> DPPAPLPLVIWHGMGDSCCNPLSMGAIKKMVEKKIPGIHVLSLEIGKTLREDVENSFFLNVNSQVTTVCQILAKDPKLQQGYNAMGFSQGGQFLRAVAQRCPSPPMVNLISVGGQHQGVFGLPRCPGESSHICDFIRKTLNAGAYNKAIQERLVQAEYWHDPIREDIYRNHSIFLADINQERGVNESYKKNLMALKKFVMVKFLNDTIVDPVDSEWFGFYRSGQAKETI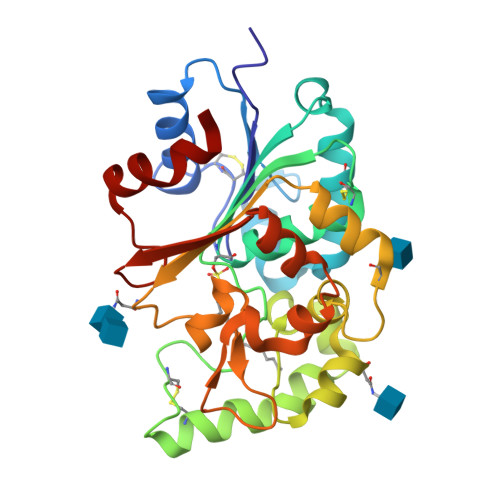PLQESTLYTQDRLGLKAMDKAGQLVFLALEGDHLQLSEEWFYAHIIPFLE> MASVHGTTYELLRRQGIDTVFGNPGSNELPFLKDFPEDFRYILALQEACVVGIADGYAQASRKPAFINLSSAAGTGNAMGALSNAWNSHSPLIVTAGQQTRAMIGVEALLTNVDAANLPRPLVKWSYEPASAAEVPHAMSRAIHMASMAPQGPVYLSVPYDDWDKDADPQSHHLFDRHVSSSVRLNDQDLDILVKALNSASNPAIVLGPDVDAANANADCVMLAERLKAPVWVAPSAPRCPFPTRHPCFRGLMPAGIAAISQLLEGHDVVLVIGAPVFRYHQYDPGQYLKPGTRLISVTCDP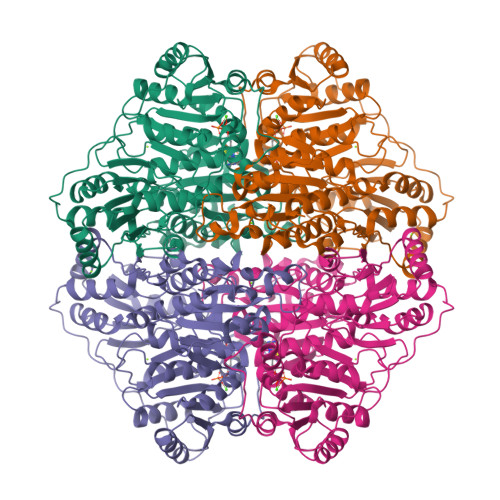LEAARAPMGDAIVADIGAMASALANLVEESSRQLPTAAPEPAKVDQDAGRLHPETVFDTLNDMAPENAIYLNESTSTTAQMWQRLNMRNPGSYYFCAAGGLGFALPAAIGVQLAEPERQVIAVIGDGSANYSISALWTAAQYNIPTIFVIMNNGTYGALRWFAGVLEAENVPGLDVPGIDFRALAKGYGVQALKADNLEQLKGSLQEALSAKGPVLIEVSTVSPVKHHHHHH> MAREAKDTVDLYDDRGNCVAEEVPIEVLSPMRNEAIQSIVNDIKRTVAVDLEGIENALQNATVGGKGMKIPGREMDVDIVDNAEAIADEIEKMIRVYQDDDTNVEPMYDGKRLLVQLPSERVKVMADPYSGTLQAGMAVVHAIIDVCEVDMWDANMVKAAVFGRYPQTI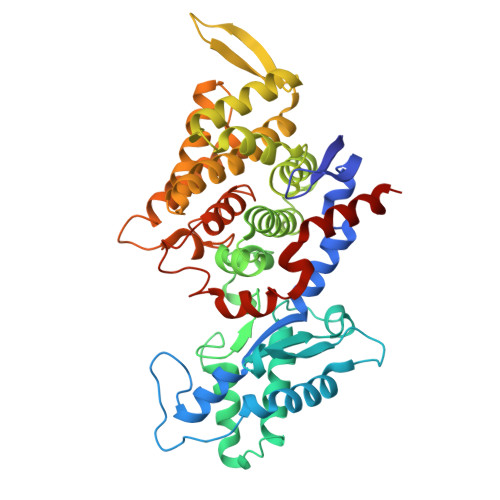DYFGGNVASMLDVPMKQEGVGYALRNIMVNHIVAATRKNTMQAVCLAATLQQTAMFEMGDALGPFERLHLLGYAYQGLNADNMVYDIVKKHGKEGTVGTVVREVVERALEDGVIEVKEELPSFKVYKANDMDLWNAYAAAGLVAAVMVNQGAARAAQGVSATILYYNDLLEYETGLPGVDFGRAEGTAVGFSFFSHSIYGGGGPGIFHGNHIVTRHSKGFAIPPVAAAMALDAGTQMFSPEVTSKLIGDVFGEIDEFREPMKYITEAAAEEAKR>[12x]GGACCCCGG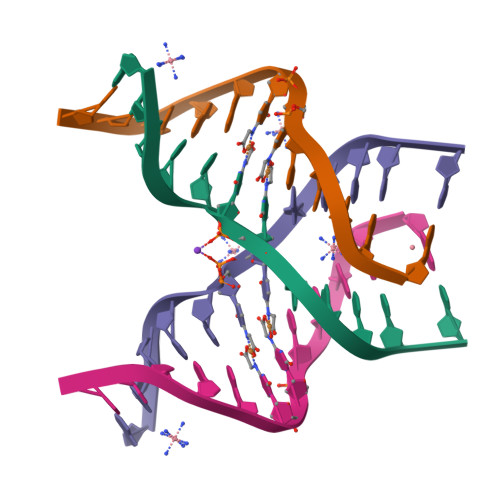TCC>[12x]GSLELIKLR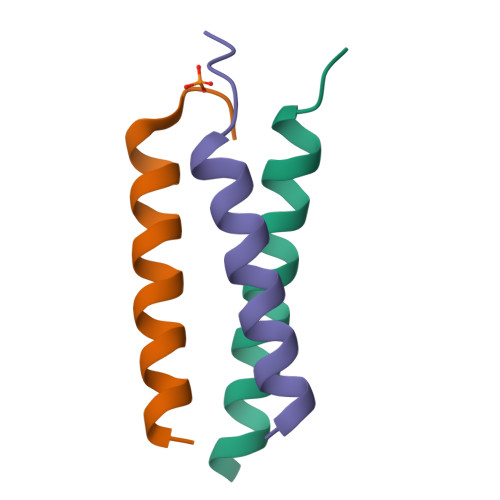IMEIEARIAKIEKDRAIL>[4x]MRFQVIVAAATITMITSYIPG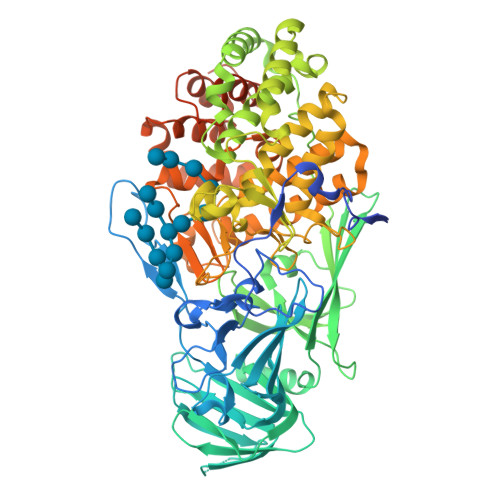VASQSTSDGDDLFVPVSNFDPKSIFPEIKHPFEPMYANTENGKIVPTNSWISNLFYPSADNLAPTTPDPYTLRLLDGYGGNPGLTIRQPSAKVLGSYPPTNDVPYTDAGYMINSVVVDLRLTSSEWSDVVPDRQVTDWDHLSANLRLSTPQDSNSYIDFPIVRGMAYITANYNNLTPQFLSQHAIISVEADEKKSDDNTSTFSGRKFKITMNDDPTSTFIIYSLGDKPLELRKQDNSNLVASKPYTGVIRVAKLPAPEFETLLDASRAVWPTGGDISARSDDNNGASYTIKWKTNSNEAPLLTYAYAHHLTSIDDSNVKRTDMTLQSATKGPMTALVGNEWTLRETELSPVEWLPLQAAPNPTTINEIMTEINKDIASNYTQETAKEDNYFSGKGLQKFAMLALILNKSDQTQLRNPELAQIALDKLKAAFLPYLQNEQADPFRYDTLYKGIVAKAGLPTSMGGTDDLSAEFGHSYYSDHHYHQGYFVVTAAIIHHLDPTWNADRLKAWTEALIRDVNNANDGDEYFAAFRNWDWFAGHSWAGGIKPDGALDGRDQESVPESVNFYWGAKLWGLATGNTPLTKLASLQLAVTKRTTYEYFWMLDGNKNRPENIVRNKVIGIYFEQKTDYTTYFGRFLEYIHGIQQLPMTPELMEYIRTPEFVSQEWDEKLGAIAPTVQSPWAGVLYLNYAIINPAEAYPALRKVQMDDGQTRSYSLYLTATRPHFFRRSLLAALARHGSTRRPSLPSSGDDDKHEDGFLLRFRRLNPFNLKHRIY> MLKGKDGVVKNASTGDSIGHLQSWALDTQRDEVSGWGMGDDAERAFTTVGRASGNFEV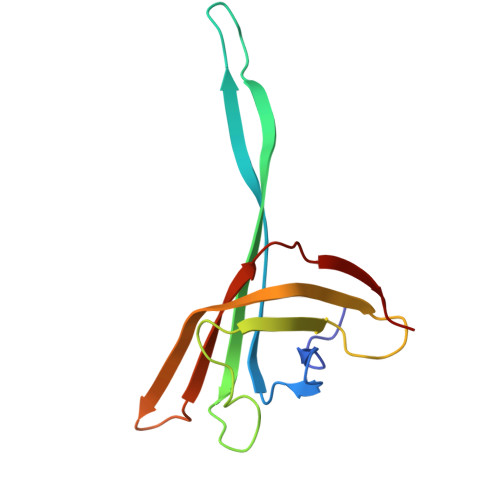YLDPADPSDDLEPGDLVDLELYPGGESTGSGYRSVAGALILSTAESASKDGIPMLTVNWRTSGALPQKATVS> NPVENYIDEVLNEVLVVPNINSSNPTTSNSAPALDAAETGHTSSVQPEDVIETRYVQTSQTRDEMSLESFLGRSGCIHESKLEVTLANYNKENFTVWAINLQEMAQIRRKFELFTYTRFDSEITLVPCISALSQDIGHITMQYMYVPPGAPVPNSRDDYAWQSGTNASVFWQHGQAYPRFSLPFLSVASAYYMFYDGYDEQDQNYGTANTNNMGSLCSRIVTEKHIHKVHIMTRIYHKAKHVKAWCPRPPRALEYTRAHRTNFKIEDRSIQTAIVTRPIITTAGPSDMY;> SPTVEACGYSDRIIQITRGDSTITSQDVANAIVAYGVWPHYLSSKDASAIDKPSQPDTSSNRFYTLRSVTWSSSSKGWWWKLPDALKDMGIFGENMFYHYLGRSGYTIHVQCNASKFHQGTLIVALIPEHQIASALHGNVNVGYNYTHPGETGREVKAETRLNPDLQPTEEYWLNFDGTLLGNITIFPHQFINLRSNNSATIIAPYVNAVPMDSMRSHNNWSLVIIPICPLETSSAINTIPITISISPMCAEFSGARAKRQ;> GLPVFITPGSGQFLTTDDFQSPCALPWYHPTKEISIPGEVKNLVEICQVDSLVPINNTDTYINSENMYSVVLQSSINAPDKIFSIRTDVASQPLATTLIGEISSYFTHWTGSLRFSFMFCGTANTTVKLLLAYTPPGIAEPTTRKDAMLGTHVIWDVGLQSTISMVVPWISASHYR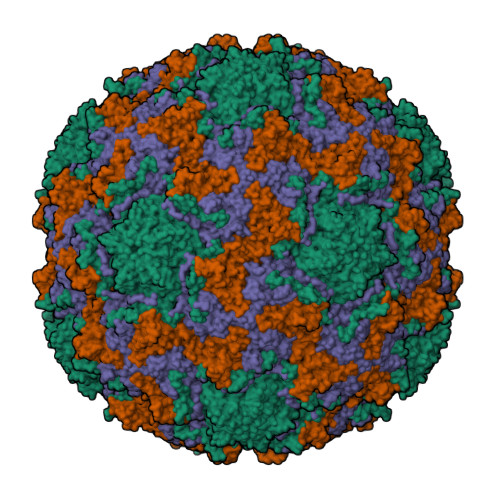NTSPGRSTSGYITCWYQTRLVIPPQTPPTARLLCFVSGCKDFCLRMARDTNLHLQSGAIAQ;> GAQVSRQNVGTHSTQNSVSNGSSLNYFNINYFKDAASNGASKLEFTQDPSKFTDPVKDVLEKGIPTLQ> MTSKPSTRNDYLPRETHNGEYTGDSPEWQLQINITNKIGGINGDIWLSRDGRSVKWCIEDQCLRQFTYNQKIIKAGYIDFEKTPDCFVVVLSDIAHVYMLKNGGSTTVCFPFQIGNAFWYANGVILERETSASFMDGGYDLKPIEFDLKHKYITLTDPMAPFGLISITNTFKGGINSASGNKTDILQDFQLVLFPSDKDKCIAVFLDRNSKVLRFYYSRILSSDQSRKGELTISSTKKTGLDAAGNSQKSGGISKDLRKFSHLTRRSTSINSNSHDFNAAERVLSGNVGNASGRTDIFALPSSCSRRSLSATLDRMGNNIAPTNRAAPSGFFDSSSANTATHSNITPVSQPMQQQQQEYLNQTATSSKDIVLTEISSLKLPDDIIFTSRRLSSILSKLKFLSLRFERREGLLIFHEPTHFCKIWLIDLLPDVLDSIPFKIYGNSPQNMIRLENLKLKEPSRIQAMYIHELLESCLILVSEGQNKEEYKACLYDPFVKITSPSKNISEELTKQNSLPSLQKLFPYPETSFTKLCFEAVKYITSPAFNISFIFLWQSAYSILLSRANDDVVGGLKMEHDAFSLVLSLLILPIPSSSAQEYQEYKEIYERDLFQHLKQDSEITSSVLPRIVIGLHLIREEYSLNVLCRNEHALLGQFLRFATAAMGWPDLWQSYYVPKMDSESKTFLHPREQNSTFFHPLDEPPSITKSLYSITENSSIPLCPFISFSRLVATDTQVELRITPRSFKILGLYELVHSPNFLPDYVLGILSSFKVDKDELQTYPLGILVPLQNILKILEDKLSEVRDNLELLDRADLQRCSAIINSIRSDSKEVLKRGQRDSYMLCKVPLAKNRSSLSKKPSDIYSILSEIVKSASQVPLDGSAMRMSNIQDDEDIDEGRSLKLNAGLIFSEDKRFTHVVSLLAYYRPTKTQFFTTKTEYAQILAQKKYFAKIMALRTCTNGVGWGAVAYATEKPISTQKWVIQPLNLISVFPDDTKITVKAPEDIAHDIVEWGQFHAGVSSGLRISKKATGITGSWIAFNKPKELDAYHGGFLLGLGLNGHLKNLEEWHIYNYLSPRNTHISIGLLLGMSSSMKGSMDSKLIKVISVHLVAFLPSGSSDLNIDLKLQTAGIIGMGMLYLNSRHKRMSDSIFAQLVSLLNVNDEMVADEEYRLAAGISLGLINLGAGQTKLRKWDSSLLGLGDDLPEDVYDSSDVEQNVMYEDLTTKLLEIVTSTYDVENDWIPENSQI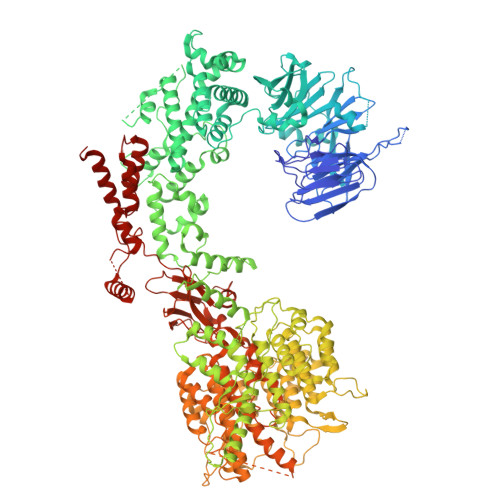GAVIAIMFLFLKSNNFGISNMLKVDLKEILKANINTRPELLMYREWASNMILWEFIGDDLSFIMKDVDIGVKFSELNTDLLPIYYTMAGRILAMGIRFASTGNLKIRNILLSLVDKFLPLYQYPGKQNLDFRLTISVINVLTNVIVVSLSMVMCASGDLEVLRRVKYLHEVASGPYSDLFQEIPSSKSDVSGVTQVTSNTNTPGNSDRERVDETAASLDDERSSNGSDISDPTAYLEDKKDIDDHYGKFISTNLALGFLFLGSGQYALNTSTLESIAFLSMSVLPTYTTPHPLQELKHFWSMAVEPRCLVIKDISTGDAVNNVPIELVVEEDVEKEEVIREISTPCLLPDFSKIKSIRVKMHGYFPLEVNFTKDYSASDFFSGGTIIYIQRKSESVFENKASFRNVEDIHVALKRKAAESKNYSRLNLKNEQGNTTSSQLVESLGIQDLTMVELDTLLSAGNNTALTDSESYNLGLLCSDKNSGDILDCQLELWYKSFGPHDE5,10,15,20-TETRAKIS(4-SULPFONATOPHENYL)-21H,23H-PORPHINE 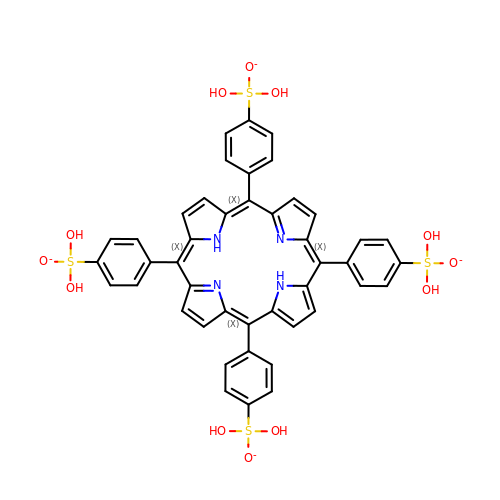| C44 H34 N4 O12 S4 | OVPFWIRROXFHGQ-LWQDQPMZSA-J>UGCGUCA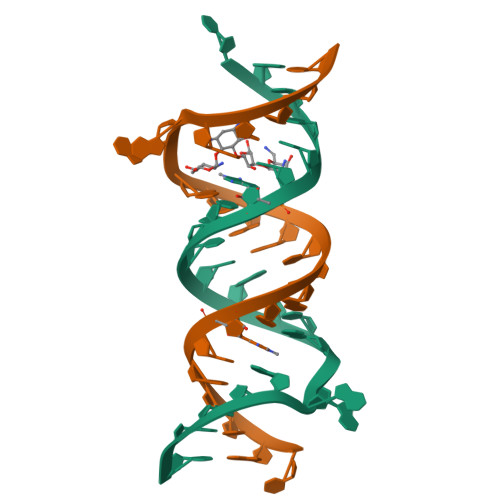CGUCGACGAAGUCGC[2x]> MSVFDRLAGFADSVTNAKQVDVSTATAQKKAEQGVTTPLVSPDAAYQMQAARTGNVGANAFEPGTVQSDFMNLTPMQIMNKYGVEQGLQLINARADAGNQVFNDSVTTRTPGEELGDIATGVGLGFVNTLGGIGALGAGLLNDDAGAVVAQQLSKFNDAVHATQSQALQDKRKLFAARNLMNEVESERQYQTDKKEGTNDIVASLSKFGRDFVGSIENAAQTDSIISDGLAEGVGSLLGAGPVLRGASLLGKAVVPANTLRSAALAGAIDAGTGTQSLARIASTVGRAAPGMVGVGAMEAGGAYQQTADEIMKMSLKDLEKSPVYQQHIKDGMSPEQARRQTASETGLTAAAIQLPIAAATGPLVSRFEMAPFRAGSLGAVGMNLARETVEEGVQGATGQLAQNIAQQQNIDKNQDLLKGVGTQAGLGALYGFGSAGVVQAPAGAARLAGAATAPVLRTTMAGVKAAGSVAGKVVSPIKNTLVARGERVMKQNEEASPVADDYVAQAAQEAMAQAPEAEVTIRDAVEATDATPEQKVAAHQYVSDLMNATRFNPENYQEAPEHIRNAVAGSTDQVQVIQKLADLVNTLDESNPQALMEAASYMYDAVSEFEQFINRDPAALDSIPKDSPAIELLNRYTNLTANIQNTPKVIGALNVINRMINESAQNGSLNVTEESSPQEMQNVALAAEVAPEKLNPESVNVVLKHAADGRIKLNNRQIAALQNAAAILKGAREYDAEAARLGLRPQDIVSKQIKTDESRTQEGQYSALQHANRIRSAYNSGNFELASAYLNDFMQFAQHMQNKVGALNEHLVTGNADKNKSVHYQALTADREWVRSRTGLGVNPYDTKSVKFAQQVALEAKTVADIANALASAYPELKVSHIKVTPLDSRLNAPAAEVVKAFRQGNRDVASSQPKADSVNQVKETPVTKQEPVTSTVQTKTPVSESVKTEPTTKESSPQAIKEPVNQSEKQDVNLTNEDNIKQPTESVKETETSTKESTVTEELKEGIDAVYPSLVGTADSKAEGIKNYFKLSFTLPEEQKSRTVGSEAPLKDVAQALSSRARYELFTEKETANPAFNGEVIKRYKELMEHGEGIADILRSRLAKFLNTKDVGKRFAQGTEANRWVGGKLLNIVEQDGDTFKYNEQLLQTAVLAGLQWRLTATSNTAIKDAKDVAAITGIDQALLPEGLVEQFDTGMTLTEAVSSLAQKIESYWGLSRNPNAPLGYTKGIPTAMAAEILAAFVESTDVVENIVDMSEIDPDNKKTIGLYTITELDSFDPINSFPTAIEEAVLVNPTEKMFFGDDIPPVANTQLRNPAVRNTPEQKAALKAEQATEFYVHTPMVQFYETLGKDRILELMGAGTLNKELLNDNHAKSLEGKNRSVEDSYNQLFSVIEQVRAQSEDISTVPIHYAYNMTRVGRMQMLGKYNPQSAKLVREAILPTKATLDLSNQNNEDFSAFQLGLAQALDIKVHTMTREVMSDELTKLLEGNLKPAIDMMVEFNTTGSLPENAVDVLNTALGDRKSFVALMALMEYSRYLVAEDKSAFVTPLYVEADGVTNGPINAMMLMTGGLFTPDWIRNIAKGGLFIGSPNKTMNEHRSTADNNDLYQASTNALMESLGKLRSNYASNMPIQSQIDSLLSLMDLFLPDINLGENGALELKRGIAKNPLTITIYGSGARGIAGKLVSSVTDAIYERMSDVLKARAKDPNISAAMAMFGKQAASEAHAEELLARFLKDMETLTSTVPVKRKGVLELQSTGTGAKGKINPKTYTIKGEQLKALQENMLHFFVEPLRNGITQTVGESLVYSTEQLQKATQIQSVVLEDMFKQRVQEKLAEKAKDPTWKKGDFLTQKELNDIQASLNNLAPMIETGSQTFYIAGSENAEVANQVLATNLDDRMRVPMSIYAPAQAGVAGIPFMTIGTGDGMMMQTLSTMKGAPKNTLKIFDGMNIGLNDITDASRKANEAVYTSWQGNPIKNVYESYAKFMKNVDFSKLSPEALEAIGKSALEYDQRENATVDDIANAASLIERNLRNIALGVDIRHKVLDKVNLSIDQMAAVGAPYQNNGKIDLSNMTPEQQADELNKLFREELEARKQKVAKARAEVKEETVSEKEPVNPDFGMVGREHKASGVRILSATAIRNLAKISNLPSTQAATLAEIQKSLAAKDYKIIYGTPTQVAEYARQKNVTELTSQEMEEAQAGNIYGWTNFDDKTIYLVSPSMETLIHELVHASTFEEVYSFYQGNEVSPTSKQAIENLEGLMEQFRSLDISKDSPEMREAYADAIATIEGHLSNGFVDPAISKAAALNEFMAWGLANRALAAKQKRTSSLVQMVKDVYQAIKKLIWGRKQAPALGEDMFSNLLFNSAILMRSQPTTQAVAKDGTLFHSKAYGNNERLSQLNQTFDKLVTDYLRTDPVTEVERRGNVANALMSATRLVRDVQSHGFNMTAQEQSVFQMVTAALATEAAIDPHAMARAQELYTHVMKHLTVEHFMADPDSTNPADRYYAQQKYDTISGANLVEVDAKGRTSLLPTFLGLAMVNEELRSIIKEMPVPKADKKLGNDIDTLLTNAGTQVMESLNRRMAGDQKATNVQDSIDALSETIMAAALKRESFYDAVATPTGNFIDRANQYVTDSIERLSETVIEKADKVIANPSNIAAKGVAHLAKLTAAIASEKQGEIVAQGVMTAMNQGKVWQPFHDLVNDIVGRTKTNANVYDLIKLVKSQISQDRQQFREHLPTVIAGKFSRKLTDTEWSAMHTGLGKTDLAVLRETMSMAEIRDLLSSSKKVKDEISTLEKEIQNQAGRNWNLVQKKSKQLAQYMIMGEVGNNLLRNAHAISRLLGERITNGPVADVAAIDKLITLYSLELMNKSDRDLLSELAQSEVEGMEFSIAYMVGQRTEEMRKAKGDNRTLLNHFKGYIPVENQQGVNLIIADDKEFAKLNSQSFTRIGTYQGSTGFRTGSKGYYFSPVAARAPYSQGILQNVRNTAGGVDIGTGFTLGTMVAGRITDKPTVERITKALAKGERGREPLMPIYNSKGQVVAYEQSVDPNMLKHLNQDNHFAKMVGVWRGRQVEEAKAQRFNDILIEQLHAMYEKDIKDSSANKSQYVNLLGKIDDPVLADAINLMNIETRHKAEELFGKDELWVRRDMLNDALGYRAASIGDVWTGNSRWSPSTLDTVKKMFLGAFGNKAYHVVMNAENTIQNLVKDAKTVIVVKSVVVPAVNFLANIYQMIGRGVPVKDIAVNIPRKTSEINQYIKSRLRQIDAEAELRAAEGNPNLVRKLKTEIQSITDSHRRMSIWPLIEAGEFSSIADAGISRDDLLVAEGKIHEYMEKLANKLPEKVRNAGRYALIAKDTALFQGIQKTVEYSDFIAKAIIYDDLVKRKKKSSSEALGQVTEEFINYDRLPGRFRGYMESMGLMWFYNFKIRSIKVAMSMIRNNPVHSLIATVVPAPTMFGNVGLPIQDNMLTMLAEGRLDYSLGFGQGLRAPTLNPWFNLTH

N4-like phages have a genome size of about 75 kb, nearly twice that of T7, and encode around 70–90 ORFs, including a characteristic large virion-associated RNA polymerase (vRNAP) unique to this family of bacterial viruses. The massive 3,500-residue vRNAP 18,19, present in 4 ± 1 copies inside the mature virion 20, is ejected into the host upon infection. In stark contrast to the N4 transcriptional program, which has been studied extensively 17, many key questions about the role of phage N4 vRNAP as an ejection protein and its part in the DNA ejectosome remain unanswered. vRNAP (gp50) consists of three predicted domains: a likely membrane-spanning N-terminal domain (NTD), a single-subunit RNA polymerase (RNAP) domain, and a large C-terminal domain of unknown function (CTD). In this study, we use a complementary top-down and bottom-up approach by determining the cryo-EM structures of both the full-length recombinantly expressed vRNAP and the fully asymmetric N4 virion tail.

Single particle analysis (SPA) of cryomicrographs revealed a heterogeneous mix of particles with two predominant and two minor populations. N4 isolated RNAP and ΔN-vRNAP tight complex were real-space refined to a model to map correlation coefficients of CC = 0.90 and 0.84, respectively. N4 RNAP domain adopts a typical single subunit RNAP (ssRNAP) fold that resembles a right hand with three subdomains: fingers, palm, and thumb. Without the CTD, the B-motif loop is folded into a beta hairpin that sits outside the active site. Thus, vRNAP can be rationalized as three globular, folded units flexibly connected by at least two extended linkers. These linkers may explain why SPA of vitrified vRNAP also captured individual RNAP and CTD domains if the two domains are separate in a “split complex”. We performed radiolabeled runoff transcriptional assays using both the full-length (FL) vRNAP and the RNAP domain alone on an 81-nt N4 native sequence ssDNA template, which contained the P1 hairpin promoter. However, the FL enzyme synthesized less RNA product as a function of time, consistent with the proposed autoinhibitory effect of the CTD.>[2x]RSPGTLPRKAGVFSDLSNQELKAVHSFLWSKKELRLQPSSTTTMAKNTVFLIEMLLPKKYHVLRFLDKGERHPVREARAVIFFGDQEHPNVTEFAVGPLPGPCYMRALSPRPGYQSSWASRPISTAEYALLYHTLQEATKPLHQFFLNTTGFSFQDCHDRCLAFTDVAPRGVASGQRRSWLIIQRYVEGYFLHPTGLELLVDHGSTDAGHWAVEQVWYNGKFYGSPEELARKYADGEVDVVVLEDPLPGGKGHDSTEEPPLFSSHKPRGDFPSPIHVSGPRLVQPHGPRFRLEGNAVLYGGWSFAFRLRSSSGLQVLNVHFGGERIAYEVSVQEAVALYGGHTPAGMQTKYLDVGWGLGSVTHELAPGIDCPETATFLDTFHY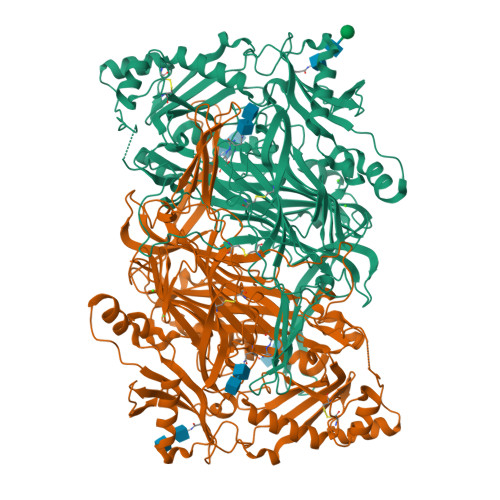YDADDPVHYPRALCLFEMPTGVPLRRHFNSNFKGGFNFYAGLKGQVLVLRTTSTVYNXDYIWDFIFYPNGVMEAKMHATGYVHATFYTPEGLRHGTRLHTHLIGNIHTHLVHYRVDLDVAGTKNSFQTLQMKLENITNPWSPRHRVVQPTLEQTQYSWERQAAFRFKRKLPKYLLFTSPQENPWGHKRSYRLQIHSMADQVLPPGWQEEQAITWARYPLAVTKYRESELCSSSIYHQNDPWDPPVVFEQFLHNNENIENEDLVAWVTVGFLHIPHSEDIPNTATPGNSVGFLLRPFNFFPEDPSLASRDTVIVWPRDNGPNYVQRWIPEDRDCSMPPPFSYNGTYRPV> GPAEVPLPQLRA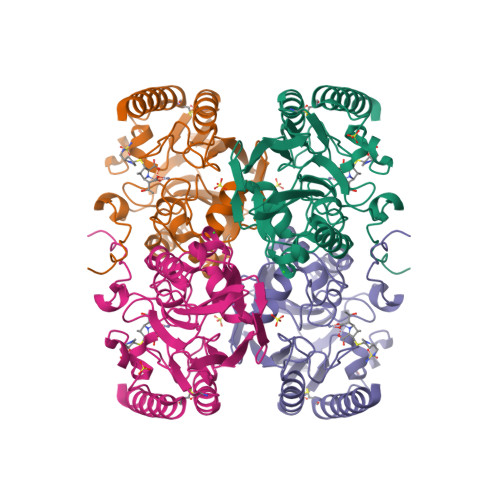YTVDASWLQPMAPLQIADHTWQIGTEDLTALLVQTPDGAVLLDGGMPQMASHLLDNMKARGVTPRDLRLILLSHAHADHAGPVAELKRRTGAKVAANAESAVLLARGGSDDLHFGDGITYPPANADRIVMDGEVITVGGIVFTAHFMAGHTPGSTAWTWTDTRNGKPVRIAYADSLSAPGYQLQGNPRYPHLIEDYRRSFATVRALPCDVLLTPHPGASNWDYAAGARAGAKALTCKAYADAAEQKFDGQLAKETAGAR>[2x]MAEQVKPAGVKPKGTVPPPKGNAPAPKANGAPGGASVIKEQDAAKMRRFLFQRTETRSTKWYQIFDTEKLDDEQVVGGHLALLGVLGFIMGIYYISGIQVFPWGAPGFHDNWFYLTIKPRMVSLGIDTYSTKTADLEAAGARLLGWAAFHFLVGSVLIFGGWRHWTHNLTNPFTGRCGNFRDFRFLGKFGDVVFNGTSAKSYKEALGPHAVYMSLLFLGWGIVMWAILGFAPIPDFQTINSETFMSFVFAVIFFALGIYWWNNPPNAAIHLNDDMKAAFSVHLTAIGYINIALGCIAFVAFQQPSFAPYYKELDKLVFYLYGEPFNRVSFNFVEQGGKVISGAKEFADFPAYAILPKSGEAFGMARVVTNLIVFNHIICGVLYVFAGVYHGGQYLLKIQLNGMYNQIKSIWITKGRDQEVQVKILGTVMALCFATMLSVYAVIVWNTICELNIFGTNITMSFYWLKPLPIFQWMFADPSINDWVMAHVITAGSLFSLIALVRIAFFAHTSPLWDDLGLKKNSYSFPCLGPVYGGTCGVSIQDQLWFAMLWGIKGLSAVCWYIDGAWIASMMYGVPAADAKAWDSIAHLHHHYTSGIFYYFWTETVTIFSSSHLSTILMIGHLVWFISFAVWFEDRGSRLEGADIQTRTIRWLGKKFLNRDVNFRFPVLTISDSKLAGTFLYFGGTFMLVFLFLANGFYQTNSPLPPPVSHAAVSGQQMLAQLVDTLMKMIA;> MAEPVENKNQAPAPGAKVPPKGAPAAPKAGAPAAPKGPVAPKAGAPAAKTGASAAKQAGKPRLASLGVTLGRSGVRQESALPYVKPKAVPPPKPAAPAAKGAPAPKGAPAAPAAKAAPGAPVAKAAPKAKKHYFIIENLCVGCGLCLDKCPPKVNAIGYKFYGDVQEGGFRCYIDQAACISCSACFSGDECPSGALIEVLPDGEVLDFSYTPPE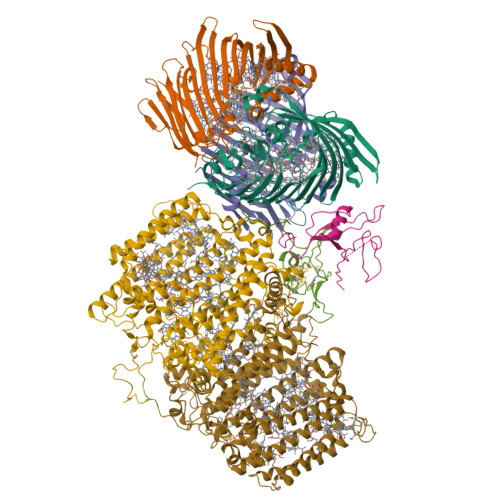RLDFDLRFLHRFHREAR;> MQPQLSRPQTASNQVRKAVSGPWSGNAVHKAEKYFITSAKRDRDGKLQIELVPASGRRKLSPTPEMIRRLIDGEIEIYILTTQPDIAIDMNKEIIDMENRYVIDFDKRGVKWTMREIPVFYHEGKGLCVELHNKIYTLDQFFK;>MALFGSNDVTTAHSDYEIVLEGGSSSWGKVKARAKVNAPPASPLLPADCDVKLNVKPLDPAKGFVRISAVFESIVDSTKNKLTIEADIANETKERRISVGEGMVSVGDFSHTFSFEGSVVNLFYYRSDAVRRNVPNPIYMQGRQFHDILMKVPLDNNDLIDTWEGTVKAIGSTGAFNDWIRDFWFIGPAFTALNEGGQRISRIEVNGLNTESGPKGPVGVSRWRFSHGGSGMVDSISRWAELFPSDKLNRPAQVEAGFRSDSQGIEVKVDGEFPGVSVDAGGGLRRILNHPLIPLVHHGMVGKFNNFNVDAQLKVVLPKGYKIRYAAPQYRSQNLEEYRWSGGAYARWVEHVCKGGVGQFEILYAQ[3x]>[2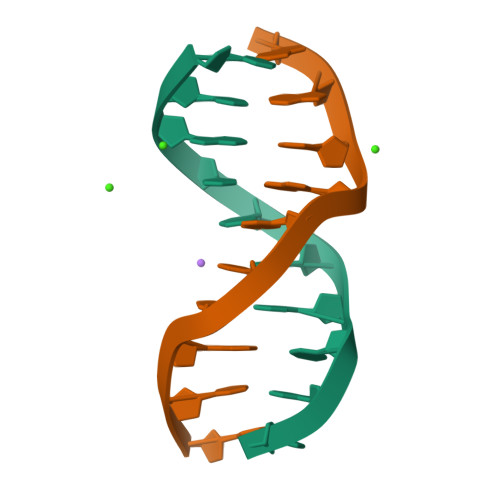x]CCGTCGACGG> MSRKRSTKPKPAAKIALKKENDQFLEALKLYEGKQYKKSLKLLDAILKKDGSHVDSLALKGLDLYSVGEKDDAASYVANAIRKIEGASASPICCHVLGIYMRNTKEYKESIKWFTAALNNGSTNKQIYRDLATLQSQIGDFKNALVSRKKYWEAFLGYRANWTSLAVAQDVNGERQQAINTLSQFEKLAEGKISDSEKYEHSECLMYKNDIMYKAASDNQDKLQNVLKHLNDIEPCVFDKFGLLERKATIYMKLGQLKDASIVYRTLIKRNPDNFKYYKLLEVSLGIQGDNKLKKALYGKLEQFYPRCEPPKFIPLTFLQDKEELSKKLREYVLPQLERGVPATFSNVKPLYQRRK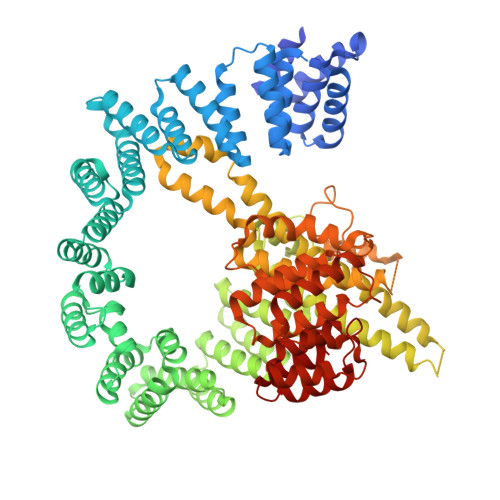SKVSPLLEKIVLDYLSGLDPTQDPIPFIWTNYYLSQHFLFLKDFPKAQEYIDAALDHTPTLVEFYILKARILKHLGLMDTAAGILEEGRQLDLQDRFINCKTVKYFLRANNIDKAVEVASLFTKNDDSVNGIKDLHLVEASWFIVEQAEAYYRLYLDRKKKLDDLASLKKEVESDKSEQIANDIKENQWLVRKYKGLALKRFNAIPKFYKQFEDDQLDFHSYCMRKGTPRAYLEMLEWGKALYTKPMYVRAMKEASKLYFQMHDDRLKRKSDSLDENSDEIQNNGQNSSSQKKKAKKEAAAMNKRKETEAKSVAAYPSDQDNDVFGEKLIETSTPMEDFATEFYNNYSMQVREDERDYILDFEFNYRIGKLALCFASLNKFAKRFGTTSGLFGSMAIVLLHATRNDTPFDPILKKVVTKSLEKEYSENFPLNEISNNSFDWLNFYQEKFGKNDINGLLFLYRYRDDVPIGSSNLKEMIISSLSPLEPHSQNEILQYYL>MDAERNLYAIVGISCRFPGANTAEQLWNVLMEQRDAITTFCPAENLGFALEENSVFVPRYGMIDALKDFEPSAYSMSDAEAQTIDPQKRVFLDVAADALADAGTSASPGNPLDPVGVFVGAATNTFLSSRDNPGSKPPGDEEPQSFANHYQQLLDCPIGTFASFKLNLTGPVVTLNTACSSALAALHLACASLSHGDCNAAVVGGVSMAYPQEGGYVTARPGGDSSAVFSPSGVCHPLDSRADGCVPADGAAALVIKRLADARADGCRVYAVIEGVAVSADGSDDKAGLGVPSSSGQSRTVEAALRRAGPQALSRLRYVEMHGSGTPWGDALEVQGLKMAFDRLSKTGAAEQSGTGRAQPEADRIYLGSNKGNCGNTEAASGLLSLIKASMALNLGVVPPLPNLAEPNPKCEFEETKFEPLGKQLALAPGDRVGVTSLGYGGSNAHVVLASAQLFGV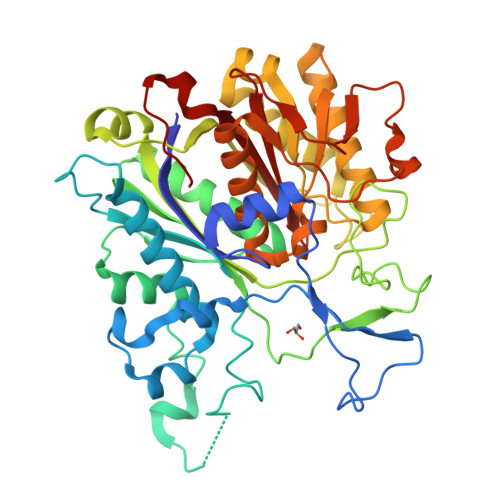EQKAFF[2x]> MANLEIGKSILAAGVLTNYHDVGEGQPVILIHGSGPGVSAYANWRLTIPALSKFYRVIAPDMVGFGFTDRPENYNYSKDSWVDHIIGIMDALE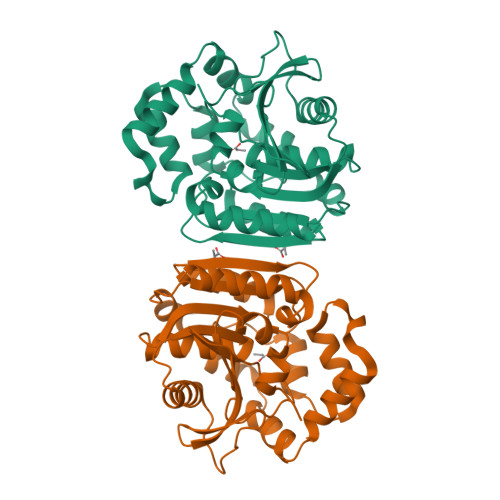IEKAHIVGNAFGGGLAIATALRYSERVDRMVLMGAAGTRFDVTEGLNAVWGYTPSIENMRNLLDIFAYDRSLVTDELARLRYEASIQPGFQESFSSMFPEPRQRWIDALASSDEDIKTLPNETLIIHGREDQVVPLSSSLRLGELIDRAQLHVFGRCGHWTQIEQTDRFNRLVVEFFNEANTPKLVGRP> SQPNATLYKMSSINADFAFNLYRRFTVETPDKNIFFSPVSISAALVMLSFGACCSTQTEIVETLGFNLTDTPMVEIQHGFQHLICSLNFPKKELELQIGNALFIGKHLKPLAKFLNDVKTLYETEVFSTDFSNISAAKQEINSHVEMQTKGKVVGLIQDLKPNTIMVLVNYIHFKAQWANPFDPSKTEDSSSFLIDKTTTVQVPMMHQMEQYYHLVDMELNCTVLQMDYSKNALALFVLPKEGQMESVEAAMSSKTLKKWNRLLQKGWVDLFVPKFSISATYDLGATLLKMGIQHAYSENADFSGLTEDNGLKLSNAAHKAVLHIGEKGTEAAGAMFLEAIPR;> SENTFLHPIIQIDRSFMLLILERSTRSILFLG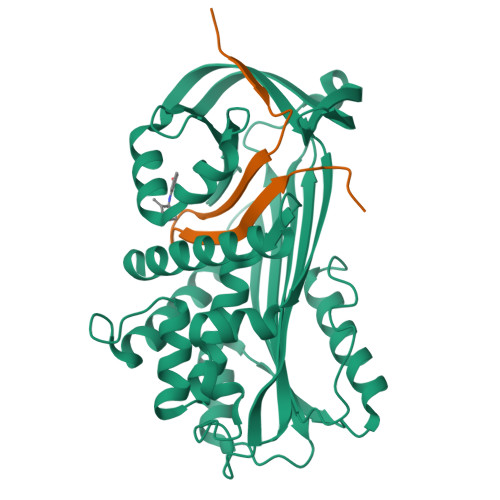KVVNPTEA>MPLNRTLSMSSLPGLEDWEDEFDLENAVLFEVAWEVANKVGGIYTVLQTKAKVTGDEWGDNYFLVGPYTEQGVRTQVELLEAPTPALKRTLDSMNSKGCKVYFGRWLIEGGPLVVLLDVGASAWALERWKGELWDTCNIGVPWYDREANDAVLFGFLTTWFLGEFLAQSEEKPHVVAHFHEWLAGVGLCLCRARRLPVATIFTTHATLLGRYLCAGAVDFYNNLENFNVDKEAGERQIYHRYCMERAAAHCAHVFTTVSQITAIEAQHLLKRKPDIVTPNGLNVKKFSAMHEFQNLHAQSKARIQEFVRGHFYGHLDFNLDKTLYFFIAGRYEFSNKGADVFLEALARLNYLLRVNGSEQTVVAFFIMPARTNNFNVETLKGQAVRKQLWDTANTVKEKFGRKLYESLLVGSLPDMNKMLDKEDFTMMKRAIFATQRQSFPPVCTHNMLDDSSDPILTTIRRIGLFNSSADRVKVIFHPEFLSSTSPLLPVDYEEFVRGCHLGVFPSYYEPWGYTPAECTVMGIPSISTNLSGFGCFMEEHIADPSAYGIYILDRRFRSLDDSCSQLTSFLYSFCQQSRRQRIIQRNRTERLSDLLDWKYLGRYYMSARHMALSKAFPEHFTYEPNEADAAQGYRYPRPASVPPSPSLSRHSSPHQSEDEEDPRNGPLEEDGERYDEDEEAAKDRRNIRAPEWPRRASCTSSTSGSKRNSVDTATSSSLSTPSEPLSPTSSLGEERN[4x];>[4x]MADQAFVTLTTNDAYAKGALVLGSSLKQHRTTRRLVVLATPQVSDSMRKVLETVFDEVIMVDVLDSGDSAHLTLMKRPELGVTLTKLHCWSLTQYSKCVFMDADTLVLANIDDLFDREELSAAPDPGWPDCFNSGVFVYQPSVETYNQLLHLASEQGSFDGGDQGILNTFFSSWATTDIRKHLPFIYNLSSISIFSYLPAFKVFGASAKVVHFLGRVKPWNYTYDPKTKSVKSEAHDPNMTHPEFLILWWNIFTTNVLPLLQQFGLVKDTCSYVNVEDVSGAISHLSLGEIPAMAQPFVSSEERKERWEQGQADYMGADSFDNIKRKLDTYLQ

Glycogen is synthesised through the cooperative action of three enzymes: glycogenin (GN), glycogen synthase (GS) and glycogen branching enzyme (GBE). GS is the rate limiting enzyme in glycogen biosynthesis and as such its activity is tightly regulated. GS is inactivated by covalent phosphorylation at numerous N- and C-terminal sites, and is allosterically activated by glucose-6-phosphate (G6P) binding and/or dephosphorylation. Here, we report the structural and functional analysis of the full-length human GS-GN complex and the cryo-EM structure of phosphorylated human GS.

The 3D reconstruction revealed a tetrameric arrangement of human GS in agreement with the crystal structures of the C. elegans GS and yeast GS enzymes, with root mean square deviation (RMSD) values of 1.1 Å (between 484 Cα atom pairs) and 0.9 Å (between 522 Cα atom pairs) respectively. Density for the C-terminal GS interacting region of GN allows for model building of residues 300–332 (human GN34). Four GN peptides bind to the GS tetramer, and these residues form a helix-turn helix, where the first helix is denoted binding helix 1 (BH1) and the second as BH2. We were able to build a model for the N-terminus starting from residue 13, and of the C-terminus up to residue 625, and then from 630–639 (chain A/C) and 630–642 (chain B/D), that could help understand the mechanisms of GS inactivation. The N- and C-terminal tails of each GS protomer lie almost parallel to each other, and travel side by side along the GS tetrameric core to reach the centre. The C-terminal tail from chain B continues to travel further across the regulatory helices than chain A, prior to traversing away from the core. This allows chain B to engage with the regulatory helices α22, specifically phosphorylated S641 interacting with residues R588 and R591, which come from two GS protomers to form a positively charged pocket we have termed the “arginine cradle”. S641 is a major phosphorylation site involved in the regulation of GS activity, and interaction of pS641 with the arginine cradle in helix α22 shows the mechanism of inactivation of human GS through constraining the GS tetramer in a “tense state”. Interestingly, these “spike” regions were present in all the refined classes, and suggests that GS exists as a continuum of structures with a core inactive tetramer and “dynamic spikes” buttressed on either side, thus preventing GS from adopting an open, active conformation. Each human GS protomer shows a closed conformation of its active site, and a regulatory loop that only becomes ordered upon G6P binding is disordered in the human structure. However, our EM density maps show no extra density within the G6P binding site.3-bromanyl-~{N}-methyl-2~{H}-pyrazolo[4,3-d]pyrimidin-7-amine | C6 H6 Br N5 | 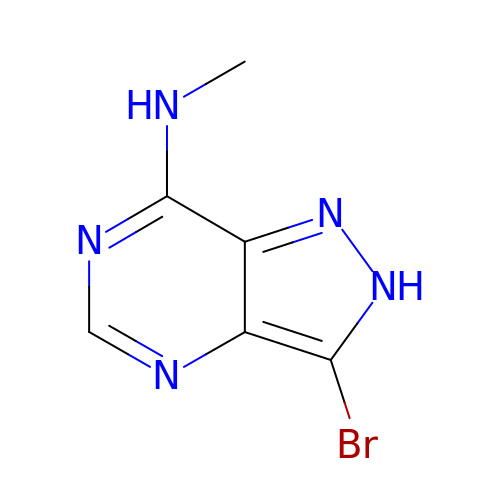AOVWLHFPQGGIAW-UHFFFAOYSA-N> GSHMSETASWQPSASIPNLLKRAAIMAEIRRFFADRGVLEVETPCMSQATVTDIHLVPFETRFVGPGHSQGMNLWLMTSPEYHMKRLLVAGCGPVFQLCRSFRNEEMGRYHNPEFTMLEWYRPHYDMYRLMNEVDDLLQQVLDCPAAESLSYQQAFLRYLEIDPLSADKTQLREVAAKLDLSNVADTEEDRDTLLQLLFTFGVEPNIGKEKPTFVYHFPASQASLAQISTEDHRVAERFEVYYKGIELANGFHELTDARE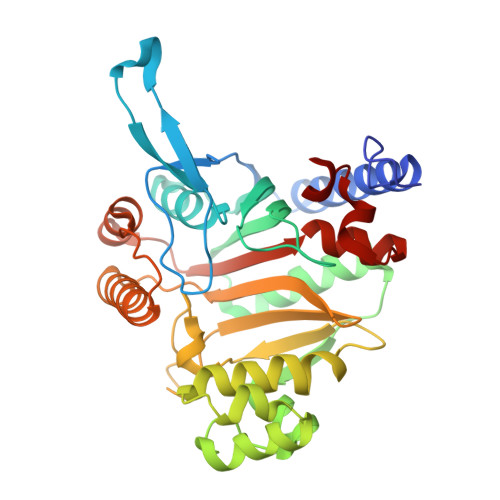QQQRFEQDNRKRAARGLPQHPIDQNLIEALKVGMPDCSGVALGVDRLVMLALGAETLAEVIAFSVDRA>GCQDDDLEDQSIFDASEKEKSEFDRWLLENYVNPYNIDFKYRMEHIESDYTHNLVPTDFWLSVKLAKIVKHCWLEAYDEVGGLDFTRACAPKVIHLIGSASWDKGTYTLGTAEGGLKVTLYMGNWLDLTNVDRMNEYYFKVMHHEFAHILHQKKNYPVDYDKISAGNYTPTGWQNRKLAEVAPLGFVTPYAGSKPSEDIAEVTACFLTYPEAQWENVMTLAGEKGKPIIDQKLAMVKKYMKDSWQVDLDLLRKVIARRTNEIS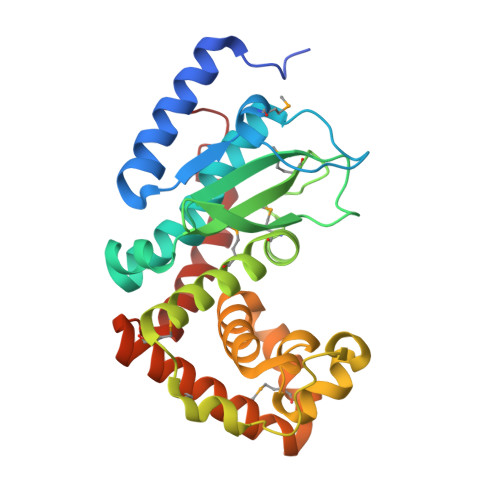ELDLDHIY[2x]> QSTEASPKRSDGTPFPWNKIRLPEYVIPVHYDLLIHANLTTLTFWGTTKVEITASQPTSTIILHSHHLQISRATLRKGAGERLSEEPLQVLEHPRQEQIALLAPEPLLVGLPYTVVIHYAGNLSETFHGFYKS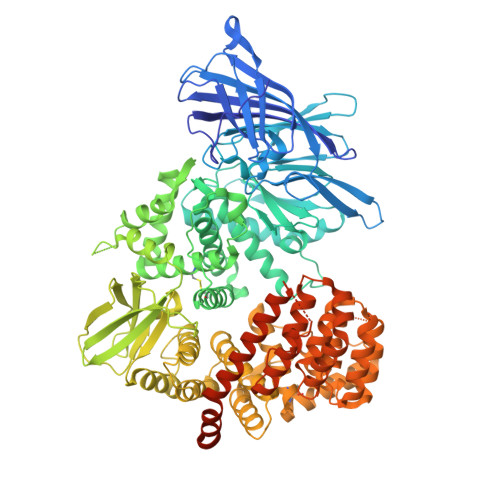TYRTKEGELRILASTQFEPTAARMAFPCFDEPAFKASFSIKIRREPRHLAISNMPLVKSVTVAEGLIEDHFDVTVKMSTYLVAFIISDFESVSKITKSGVKVSVYAVPDKINQADYALDAAVTLLEFYEDYFSIPYPLPKQDLAAIPDFQSGAMENWGLTTYRESALLFDAEKSSASSKLDITMTVAHELAHQWFGNLVTMEWWNDLWLNEGFAKFMEFVSVSVTHPELKVGDYFFGKCFDAMEVDALNSSHPVSTPVENPAQIREMFDDVSYDKGACILNMLREYLSADAFKSGIVQYLQKHSYKNTKNEDLWDSMASICPTDGVKGMDGFCSRSQHSSSSSHWHQERVDVKTMMNTWTLQRGFPLITITVRGRNVHMKQEHYMKGSDGAPDTGYLWHVPLTFITSKSDMVHRFLLKTKTDVLILPEEVEWIKFNVGMNGYYIVHYEDDGWDSLTGLLKGTHTAVSSNDRASLINNAFQLVSIGKLSIEKALDLSLYLKHETEIMPVFQGLNELIPMYKLMEKRDMNEVETQFKAFLIRLLRDLIDKQTWTDEGSVSERMLRSELLLLACVHNYQPCVQRAEGYFRKWKESNGNLSLPVDVTLAVFAVGAQSTEGWDFLYSKYQFSLSSTEKSQIEFALCRTQNKEKLQWLLDESFKGDKIKTQEFPQILTLIGRNPVGYPLAWQFLRKNWNKLVQKFELGSSSIAHMVMGTTNQFSTRTRLEEVKGFFSSLKENGSQLRCVQQTIETIEENIGWMDKNFDKIRVWLQSEKLEHDPEADATGLERMLESRGPFEQKLISEEDLNMHTEHHHHHH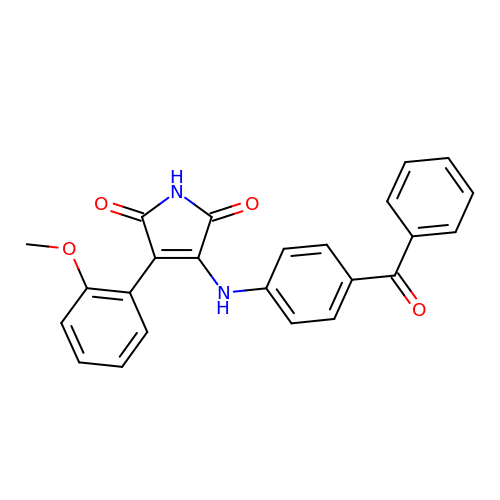3-(2-methoxyphenyl)-4-[[4-(phenylcarbonyl)phenyl]amino]pyrrole-2,5-dione | C24 H18 N2 O4 | CXBAABOAUNPLDL-UHFFFAOYSA-N> MRIGRSRRRALSLLAGVFGCAAVAATPALALPKGKPEEGGFSAERLKRLDDHMQTMVDRGQIAGGVTVLARHGRVVQARAFGRR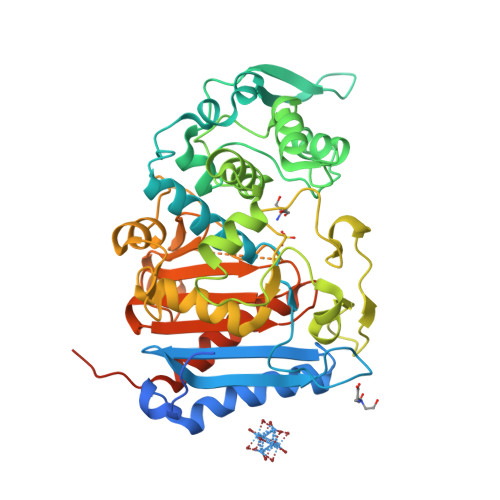VLGGDPMPMDAIFRIRSETKPVTGVAMMMLYEQGLWRLDDPVSLHIPEFANLRVAKGVDETGQPILTPVSRSPTMRELMTHTAGFAYGLANDPSSPADQAYYRAEVLQSASLTDLVQKVSGLPMFAEPGQLWRYSVAADIQGYIVEKLSGQSLPVFMQERIFTPLGMKDTAFYVPEEKQARLAALYDGDPATGQLVPAVEGAWRDVSKPPAAPLGGGGLVSTAGDFARFAQMILNKGELDGVRILKPETVALMTQNHLPEGFVVTTNGTAGVLAPAARPFPFAAGMGYGIDMAVAVDPAASGAPVGPGTVSWGGSAGTWFWIDPANNLFFVGMIQRLGGVGPGLDAQSRTLVYQALERPPMPPVQVSAKAPVRPTVSRKLAAALE>MGSSHHHHHHGSMYIAIDGDDVGRKITSSYLSNSEERLTYISNKLNDTTKKISK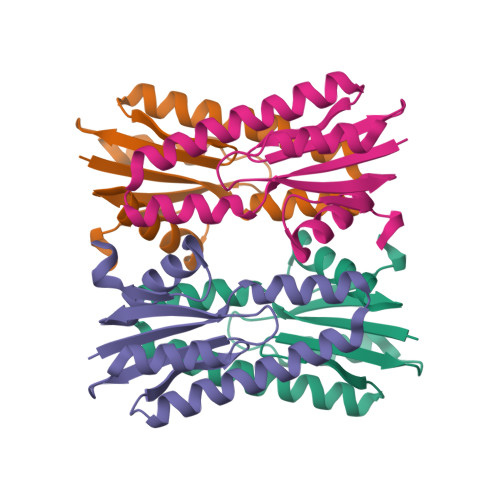MLLSNGFEIIFQAADGVTAKTDNEVNLNFVFDKIKSYSFDEITFSAGVGANLREAYVALLNSKSNGKNMISIYKDIL[4x]> SMQEEDTFRELRIFLRNVTHRLAIDKRFRVFTKPVDPDEVPDYVTVIKQPMDLS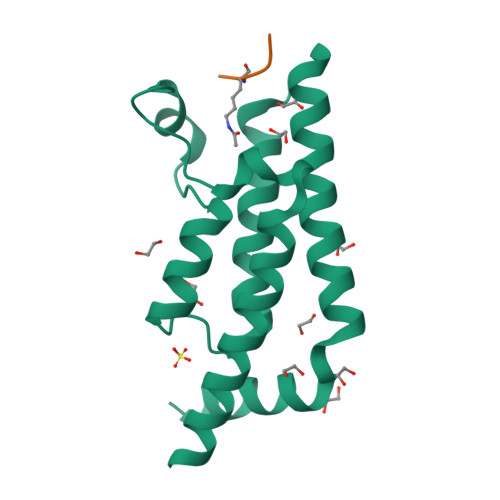SVISKIDLHKYLTVKDYLRDIDLICSNALEYNPDRDPGDRLIRHRACALRDTAYAIIKEELDEDFEQLCEEIQESR;> RGKGGKGLGKGGAY Herein we report the first X-ray crystal structures of mixed chirality α-helices in short peptides comprising only natural residues as the example of a stapled bicyclic and a linear membrane disruptive amphiphilic antimicrobial peptide (AMP) containing seven l- and four d-residues, as complexes of fucosylated analogs with the bacterial lectin LecB. The mixed chirality α-helices are superimposable onto the homochiral α-helices and form under similar conditions as shown by CD spectra and MD simulations but non-hemolytic and resistant to proteolysis. To get a direct insight into the structure of AMBP bp65/bp69 and their linear analogs ln65/ln69, we performed several crystallization studies using either the compounds themselves or their racemates to be crystallized as pure compounds, or their fucosylated derivatives of both mirror image peptides as complexes with the P. aeruginosa lectin LecB. While previous reports of similar mixed chirality AMPs concluded on either unordered conformations or helical conformations appearing in a membrane environment based on deconvolution of FTIR spectra, here we reported X-ray crystallographic evidence of short mixed chirality helices consisting of only natural residues existing as helix bundles within the protein environment of a lectin and almost perfectly superimposable with their parent homochiral α-helices. These direct observations unequivocally demonstrate that the α-helical fold with only natural residues can sometimes tolerate multiple stereochemical inversions without significant conformational changes.

In all four individually resolved homochiral bicyclic structures, the peptides were present in almost perfectly superimposable conformations featuring nine of the eleven residues forming two full turns of a right-handed α-helix including the pair of stapling cysteines (ESI†). The two N-terminal residues and the N-terminal toluoyl double staple formed a turn conformation. In all four cases the α-helical fold resulted in an amphiphilic arrangement of hydrophobic and cationic residues corresponding to the helix-wheel model and explaining the membrane disruptive activities discussed above. Remarkably, the ten crystallographically non-equivalent stapled bicyclic α-helices observed in the X-ray structures of the homochiral rac-bp65 and bp70, and the mixed chirality bp71·LecB complex were essentially superimposable, with RMSD < 0.6 Å for the peptide backbones.

> XHALYACIRCYAX> AYSLNNWNKPIKNSVTTKQWMSALPDTTNLAALSIPGTHDTMSYNGDITWTLTKPLAQTQTMSLYQQLEAGIRYIDIRAKDNLNIYHGPIFLNASLSGVLETITQFLKKNPKETIIMRLKDEQNSNDSFDYRIQPLINIYKDYFYTTPRTDTSNKIPTLKDVRGKILLLSENHTKKPLVINSRKFGMQFGAPNQVIQDDYNGPSVKTKFKEIVQTAYQASKADNKLFLNHISATSLTFTPRQYAAALNNKVEQFVLNLTSEKVRGLGILIMDFPEK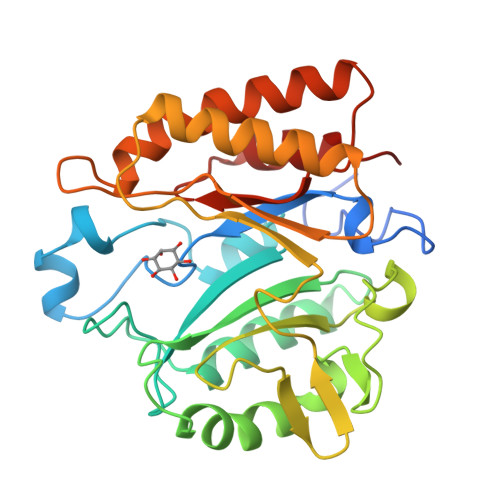QTIKNIIKNNKFN>MNYFIVEVSEQEVKREKEKARELRRSQWWKNRIARGICHYCGEIFPPEELTMDHLVPVVRGGKSTRGNVVPACKECNNRKKYLLPVEWEEYLDSLESEPSDGEGLEHHHHH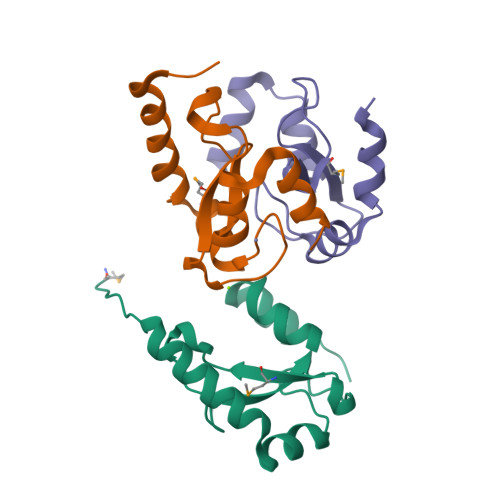H[3x]>MSSRVPILKVDDYWVVAIEETLHDQSVIQFKEELLHNITGVAGKGLVIDISALEVVDEFVTRVLIEISRLAELLGLPFVLTGIKPAVAITLTEMGLDLRGMATALNLQKGLDKLKNLARMEQ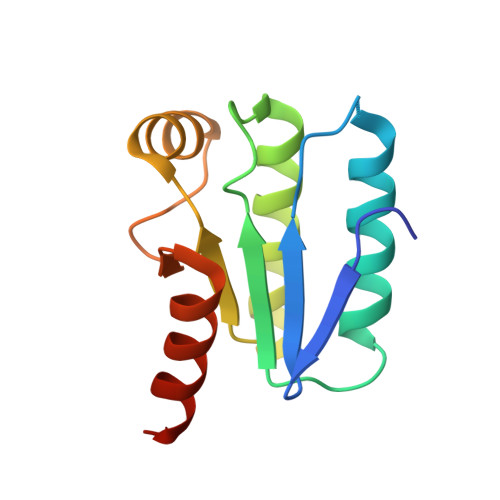R[2x]> MNISRMNVDFGNSMYMNLIDGYFFELPTNVVEISKEAAEGKFTSIVEDPADLKDRLLVSTVID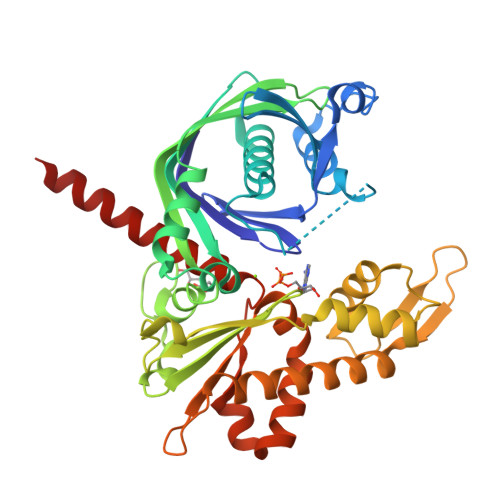ETERYFLVGELAEPEVLGNQHIKKLHNKVESHIPYVTFLAATAYYQALKGKREDNEVTIEYFQTMLPIWLLKKLDKFSEMQKRMASKFLGTHQVKVLTLGLEKELTIKVEDAACRIESEVARWAIKKNFDLEDKDYAEQFKNYDVVFCDLGGGTDDLVLLPAGLKPPKSRDSFVSNTAPFLAHLEKLRKEKLLEHFDSVRELEKFIYSNIGKTKMERRDGNTGQKFDLTDIIKKSLKEYTEIKIAQAENTFPAPKDKVYKYLYFGGVGEVLEESISVVTEERYGRDISESNHIVAEDARLLNLYGLEVLSRAEQVKKQANEKEAQ>DPATCEKEAQFVKQELIGQPYTDAVANALQSNPIRVLHPGDMITMEYIASRLNI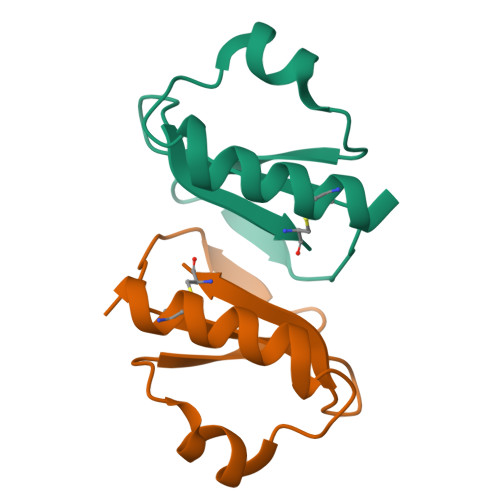QVNENNEIISAHCA[2x]>[3x]MDFSKLPKILDEDKESTFGYVHGVSGPVVTACDMAGAAMYELVRVGHSELVGEIIRLEGDMATIQVYEETSGVSVGDPVLRTGKPLSVELGPGIMGAIFDGIQRPLSDISSQTQSIYIPRGVNVSALSRDIKWDFTPCKNLRVGSHITGGDIYGIVSENSLIKHKIMLPPRNRGTVTYIAPPGNYDTSDVVLELEFEGVKEKFTMVQVWPVRQVRPVTEKLPANHPLLTGQRVLDALFPCVQGGTTAIPGAFGCGKTVISQSLSKYSNSDVIIYVGCGERGNEMSEVLRDFPELTMEVDGKVESIMKRTALVANTSNMPVAAREASIYTGITLSEYFRDMGYHVSMMADSTSRWAEALREISGRLAEMPADSGYPAYLGARLASFYERAGRVKCLGNPEREGSVSIVGAVSPPGGDFSDPVTSATLGIVQVFWGLDKKLAQRKHFPSVNWLISYSKYMRALDEYYDKHFTEFVPLRTKAKEILQEEEDLAEIVQLVGKASLAETDKITLEVAKLIKDDFLQQNGYTPYDRFCPFYKTVGMLSNMIAFYDMARRAVETTAQSDNKITWSIIREHMGDILYKLSSMKFKDPLKDGEAKIKSDYAQLLEDMQNAFRSLED;>MALRAMRGIVNGAAPELPVPTGGPAVGAREQALAVSRNYLSQPRLTYKTVSGVNGPLVILDHVKFPRYAEIVHLTLPDGTKRSGQVLEVSGSKAVVQVFEGTSGIDAKKTSCEFTGDILRTPVSEDMLGRVFNGSGKPIDRGPVVLAEDFLDIMGQPINPQCRIYPEEMIQTGISAIDGMNSIARGQKIPIFSAAGLPHNEIAAQICRQAGLVKKSKDVVDYSEENFAIVFAAMGVNMETARFFKSDFEENGSMDNVCLFLNLANDPTIERIITPRLALTTAEFLAYQCEKHVLVILTDMSSYAEALREVSAAREEVPGRRGFPGYMYTDLATIYERAGRVEGRNGSITQIPILTMPNDDITHPIPDLTGYITEGQIYVDRQLHNRQIYPPINVLPSLSRLMKSAIGEGMTRKDHADVSNQLYACYAIGKDVQAMKAVVGEEALTSDDLLYLEFLQKFERNFIAQGPYENRTVFETLDIGWQLLRIFPKEMLKRIPQSTLSEFYPRDSAKH[3x];> MSGKDRIEIFPSRMAQTIMKARLKGAQTGRNLLKKKSDALTLRFRQILKKIIETKMLMGEVMREAAFSLAEAKFTAGDFSTTVIQNVNKAQVKIRAKKDNVAGVTLPVFEHYHEGTDSYELTGLARGGEQLAKLKRNYAKAVELLVELASLQTSFVTLDEAIKITNRRVNAIEHVIIPRIERTLAYIITELDEREREEFYRLKKIQEKKKILKEKSEKDLEQRRAAGEVLEPANLLAEEKDEDLLFE;>MALSDADVQKQIKHMMAFIEQEANEKAEEIDAKAEEEFNIEKGRLVQTQRLKIMEYYEKKEKQIEQQKKIQMSNLMNQARLKVLRARDDLITDLLNEAKQRLSKVVKDTTRYQVLLDGLVLQGLYQLLEPRMIVRCRKQDFPLVKAAVQKAIPMYKIATKNDVDVQIDQESYLPEDIAGGVEIYNGDRKIKVSNTLESRLDLIAQQMMPEVRGALFGANANRKFLD[3x];>[3x]MASQSQGIQQLLQAEKRAAEKVSEARKRKNRRLKQAKEEAQAEIEQYRLQREKEFKAKEAAALGSRGSCSTEVEKETQEKMTILQTYFRQNRDEVLDNLLAFVCDIRPEIHENYRING;> MAGRGKLIAVIGDEDTVTGFLLGGIGELNKNRHPNFLVVEKDTTINEIEDTFRQFLNRDDIGIILINQYIAEMVRHALDAHQQSIPAVLEIPSKEHPYDAAKDSILRRARGMFTAEDLR;>[3x]MSFIKVGIKMGGLTSEQYHSQVVGKIGYIARCMQTIDPENNLKKIREDYQDVLIWAEKNYRFEEILEASKSGKCPNDLDALSRRSLILQELLRLVSSISPFKMKLDLIESQYEKMKQHVNLWKSDYHVKLNQLNQLTDYLKNAAPTPKNNFLRAMTSVLQMQIAQY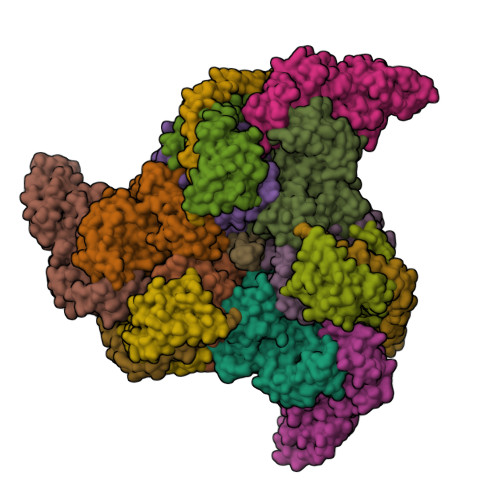GITEDNEGINQLFKLGLHLLAMANEKIDEQYHLFKGYVKDQPEESPFEGILPAEDQKILVKTMIDYAMPKLSSKVLQDKLSALSSSDVLTKTLLDSIDRIVKENEKLNALSKVKLGKFGLDIREIEVIYSQALKISPQDALQYTAQQCDAQLLSMAFPDSQNYIIESISNKKVKTIAELIHSKEFIYQIIKTEVFKQVDPNEKIRLQAATELYQLLGRIMDKQINLFTKMNLEQINEYIQTKTKAILDKIPERVELLTFMGFEIPTFKGIETLMTDISHSQDNETLAIAQEFYTNIKNAKNQLLGDKLIEDITPQDVEKFFNQCSQYGSEAAEKLADNRPVLTKIADILTAIARWAISLIGFNTPPQFLAPTRTCVDQVSDEITKIKLKLEDTLGSLQKVQEESLSL> HADEVWPGLYLGDQDMANNRRELRRLGITHVLNASHSRWRGTPEAYEGLGIRYLGVEAHDSPAFDMSIHFQTAADFIHRALSQPGGKILVHCAVGVSRSATLVLAYLMLYHHLTLV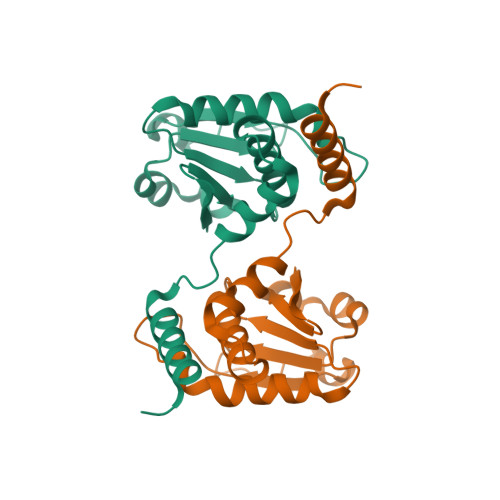EAIKKVKDHRGIIPNRGFLRQLLALDRRLRQGLEA>HHHHHHTREVVVVSGVRTAIGTFGGSLKDVAPAELGALVVREALARAQVSGDDVGHVVFGNVIQTEPRDMYLGRVAAVNGGVTINAPALTVNRLCGSGLQAIVSAAQTILLGDTDVAIGGGAESMSRAPYLAPAARWGARMGDAGLVDMMLGALHDPFHRIHMGVTAENVAKEYDISRAQQDEAALESHRRASAAIKAGYFKDQIVPVVSKGRKGDVTFDTDEHVRHDATIDDMTKLRPVFVKENGTVTAGNASGLNDAAAAVVMMERAEAERRGLKPLARLVSYGHAGVDPKAMGIGPVPATKIALERAGLQVSDLDVIEANEAFAAQ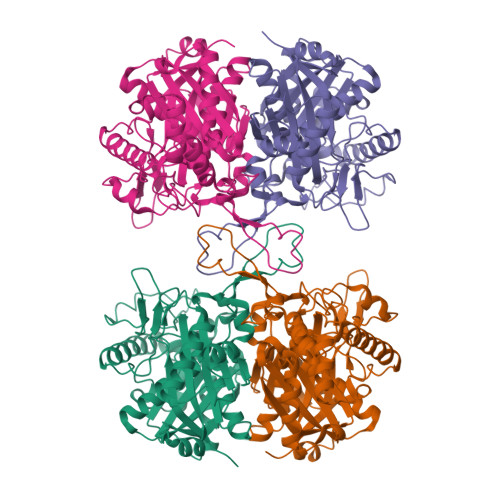ACAVTKALGLDPAKVNPNGSGISLGHPIGATGALITVKALHELNRVQGRYALVTMCIGGGQGIAAIFERI[2x]> MADDWKPQILAIICNWCSYAGADLAGGARIQYPPTVRAIRVMCTGRVDMLFILKAFVE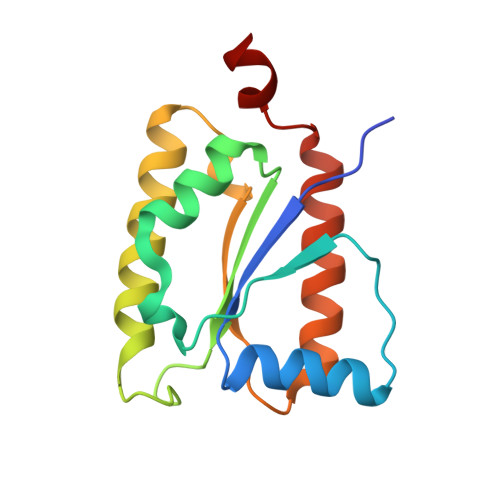GADGVLVSGCHFGDCHYLEGNYKAAKRMFMIKNLLRNIGLDDRRFRMTFVSASEGAKWGMVMEDVTNTIKELGPSPIKEFKK>YKDDDDKLHSQANLMRLKSDLFNRSPMYPGPTKDDPLTVTLGFTLQDIVKADSSTNEVDLVYYEQQRWKLNSLMWDPNEYGNITDFRTSAADIWTPDITAYSSTRPVQVLSPQIAVVTHDGSVMFIPAQRLSFMCDPTGVDSEE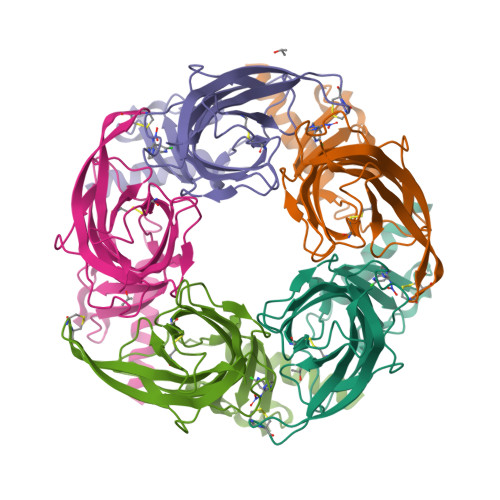GATCAVKFGSWVYSGFEIDLKTDTDQVDLSSYYASSKYEILSATQTRQVQHYSCCPEPYIDVNLVVKFRERRAGNGFFRNLFD[5x]>[3x]MIYGILSKNLGMPTPTFLVCPDVVKFENVGQIAVVNGMVYLGGSVGIDKSGTLHKGLEEQTRQTFDNIRKCLEYANSGLDYIVSLNIFLSTSLSDSEEARFNELYREV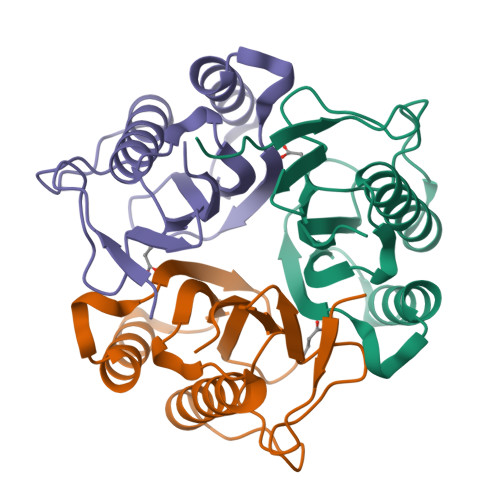FCVPATRPCRCCVRAQLQEGLLVEVVNVVAAQK> VPATLPQLTPTLVSLLEVIEPEVLYAGYDSSVPDSTWRIMTTLNMLGGRQVIAAVKWAKAIPGFRNLHLDDQMTLLQYSWMYLMAFALGWRSYRQSSANLLCFAPDLIINEQRMTLPGMYDQCKHMLYVSSELHRLQVSYEEYLCMKTLLLLSSVPKDGLKSQELFDEIRMTYIKELGKAIVKREGNSSQNWQRFYQLTKLLDSMHEVV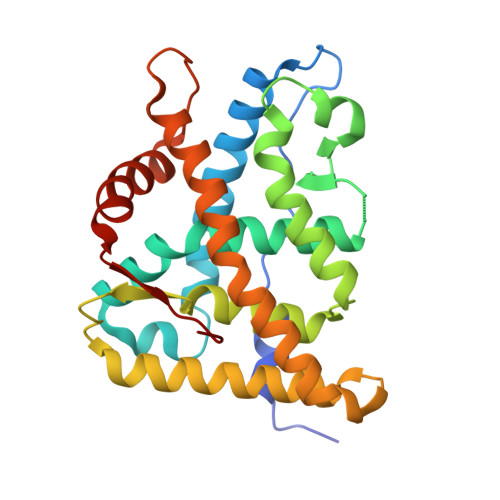ENLLNYCFQTFLDKTMSIEFPEMLAEIITNQIPKYSNGNIKKLLFHQK>QDYNLVWQDEFDDGIGPDWVFETGMGYNGWGNNELQYYRRENAAVENGNLVITAKHENFGGAQYTSARMKTQGRKSFKYGKIEARIALPSGQGLWPAFWMLGNNITSVSWPACGEIDIMSRINNALQTHGTIHWSDQNGDHASYGDDVGVSDPGQYHIYSVEWDANSIKWFVDGQQFNEVDISNGVNGTGEFQNEFFILLNMAVGGDWPGFDVDQSKLP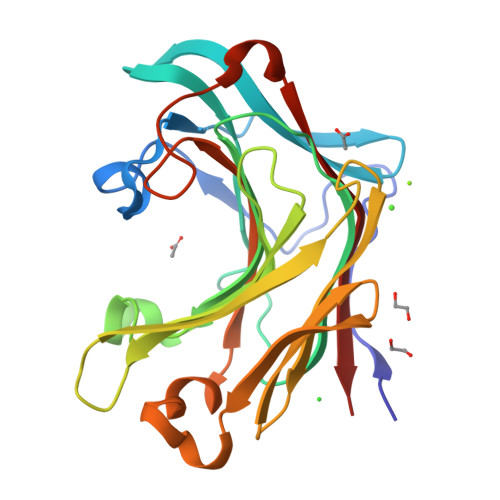AQMLVDYVRVYQKG[2x]5-Amino-1-Phenylpyrazole-4-Carboxamide 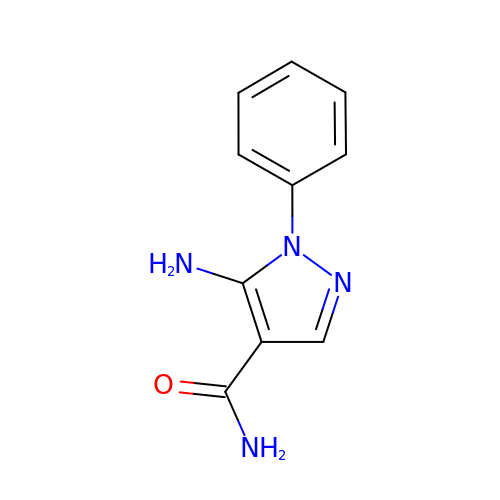| C10 H10 N4 O | UBKSUPKIDNXMMC-UHFFFAOYSA-N>TPTDKHGGSDTRCPLMVKILDAVKGTPAGSVALKVSQKTADGG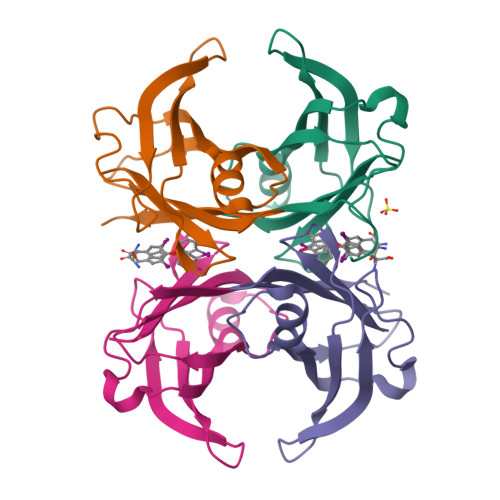WTQIATGVTDATGEIHNLITEQQFPAGVYRVEFDTKAYWTNQGSTPFHEVAEVVFDAHPEGHRHYTLALLLSPFSYTTTAVVSSVHE[4x]>MDYKDDDDKHHHHHHENLYFQGGMKHGIYYAYWEQEWEADYKYYIEKVAKLGFDILEIAASPLPFYSDIQINELKACAHGNGITLTVGHGPSAEQNLSSPDPDIRKNAKAFYTDLLKRLYKLDVHLIGGALYSYWPIDYTKTIDKKGDWERSVESVREVAKVAEACGVDFCL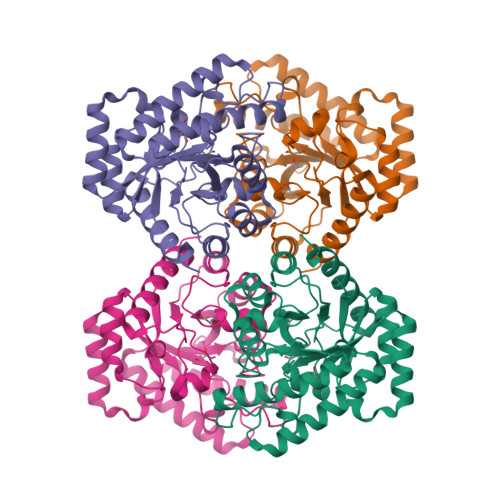EVLNRFENYLINTAQEGVDFVKQVDHNNVKVMLDTFHMNIEEDSIGGAIRTAGSYLGHLHTGECNRKVPGRGRIPWVEIGEALADIGYNGSVVMEPFVRMGGTVGSNIKVWRDISNGADEKMLDREAQAALDFSRYVLECHKHS[4x]>[2x]MQPINTS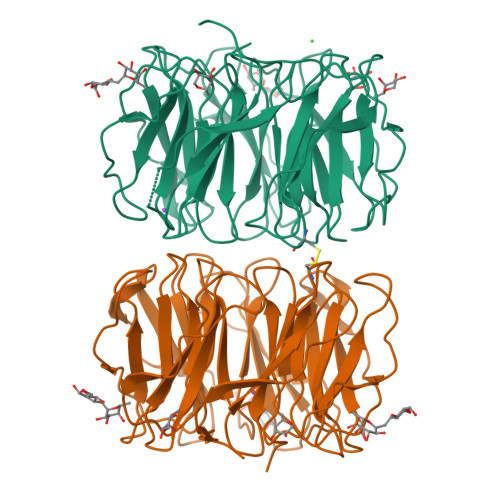NPDNTASYVKDEVEITSSTIALSEIVSVVNTSDGRLEVFGVGTDKAVWHNRQMAPHTGSPWSGWSSLKGQVTSKPVVYINTDGRLEVFARGTDNALWHIWQTATNAGWSNWQSLGGVITSNPAIYANTDGRLEVFARGADNALWHISQTTAHSGPWSSWASLNGVITSNPTVHINSDGRLEVFARGTDNALWHIWQTAPDSNLWSSWESLNGIITSDPVVIDTADGRLEVFARGADNALWHIWQTISHSGPWSGWQSLNGVITSAPAVAKNCDNRLEAFARGTDNALWHTWQTVSHSGPWSSWQSLNGVITSAPTAVRDADGRLEVFARGTDNALWLTWQTASSWSPWISLGGVLIDASAIK>[3x]GHMDVLASGEKSRMLFERTKELFPGGVNSPVRAAVKPYPFYVKRGEGAYLYTVDGARIV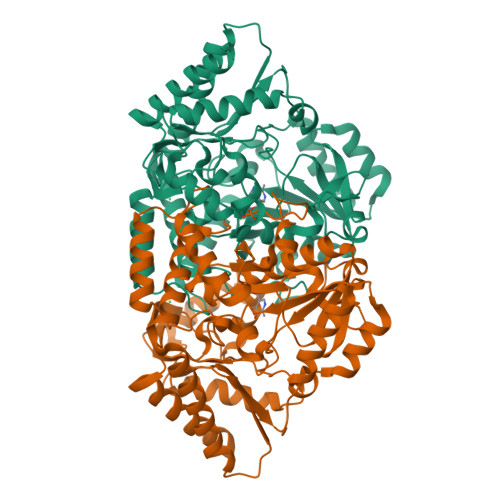DLVLAYGPLILGHKHPRVLEAVEEALARGWLYGAPGEAEVLLAEKILGYVKRGGMIRFVNSGTEATMTAIRLARGYTGRDLILKFDGCYHGSHDAVLVAAGSAAAHYGVPTSAGVPEAVARLTLVTPYNDVEALERVFAEYGDRIAGVIVEPVIANAGVIPPRREFLAALQRLSRESGALLILDEVVTGFRLGLEGAQGYFNIEGDIIVLGKIIGGGFPVGAVAGSREVMSLLTPQGKVFNAGTFNAHPITMAAGLATLKALEEEPVYSVSREAAKALEEAASEVLDRTGLPYTINRVESMMQLFIGVEEVSNAAQARKADKKFYVKLHEEMLRRGVFIAPSNLEAVFTGLPHQGEALEIAVEGLRSSLKTVLGS1-((2-HYDROXYETHOXY)METHYL)-5-(3-(BENZYLOXY)BENZYL)PYRIMIDINE-2,4(1H,3H)-DIONE 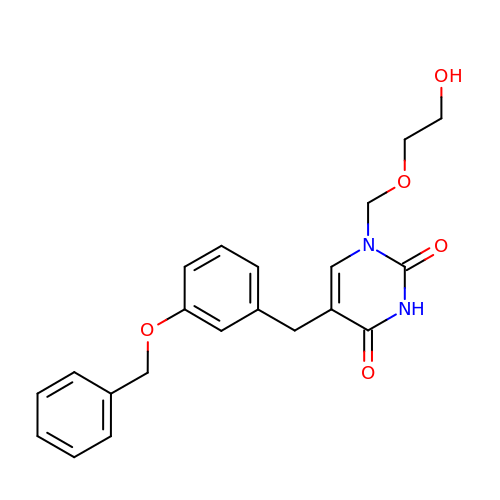| C21 H22 N2 O5 | CSXNPJKDZKLDET-UHFFFAOYSA-N>[6x]MPVFTASFQCVTLFGQPASAADAQPLLQGQRPFLHLHARRRRPCGPMLISKSPPYPASEETREWEADGQHEHTDELRETTTTMIDGIRTALRSIGEGEISISAYDTSLVALLKRLDGGDGPQFPSTIDWIVQNQLPDGSWGDASFFMMGDRIMSTLACVVALKSWNIHTDKCERGLLFIQENMWRLAHEEEDWMLVGFEIALPSLLDMAKDLDLDIPYDEPALKAIYAERERKLAKIPRDVLHSMPTTLLHSLEGMVDLDWEKLLKLRCLDGSFHCSPASTATAFQQTGDQKCFEYLDGIVKKFNGGVPCIYPLDVYERLWAVDRLTRLGISRHFTSEIEDCLDYIFRNWTPDGLAHTKNCPVKDIADTAMGFRLLRLYGYQVDPCVLKKFEKDGKFFCLHGESNPSSVTPMYNTYRA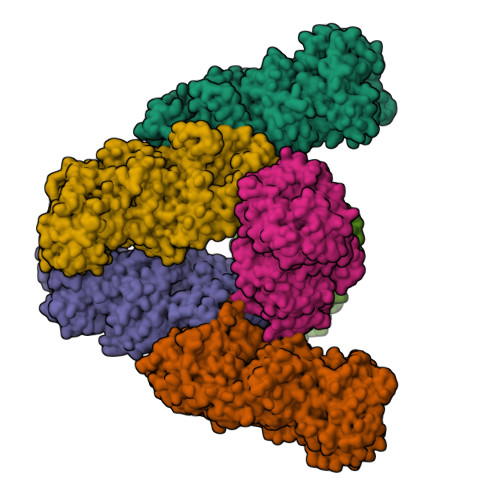SQLKFPGDDGVLGRAEVFCRSFLQDRRGSNRMKDKWAIAKDIPGEVEYAMDYPWKASLPRIETRLYLDQYGGSGDVWIGKVLHRMTLFCNDLYLKAAKADFSNFQKECRVELNGLRRWYLRSNLEKFGGTDPQTTLMTSYFLASANIFEANRAAERLGWARVALLADAVSSHFRRIGGPKNSTSNLEELISLVPFDDAYSGSLREAWKQWLMAWTAKESSQESIEGDTAILLVRAIEIFGGRHVLTGQRPDLWEYSQLEQLTSSICCKLSRRVLAQENGESTEKVEEIDQQVDLEMQELTRRVLQGCSAINRLTRETFLHVVKSFCYVAYCSPETIDSHIDKVIFQDVIEFHHHHHH>MIITSPTEARKDFYQLLKNVNNNHEPIYISGNNAENNAVIIGLEDWKSIQE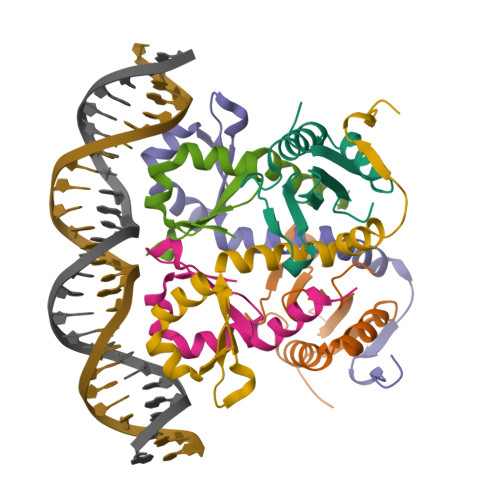TIYLESTGTMDKVREREKDNSGTTNIDDIDWDNL[8x];>[4x]HMSNYTVKIKNSAKSDLKKIKHSYLKKSFLEIVETLKNDPYKITQSFEKLEPKYLERYSRRINHQHRVVYTVDDRNKEVLILSAWSHYD4-[(4-{[(2-AMINO-4-OXO-3,4-DIHYDROQUINAZOLIN-6-YL)METHYL]AMINO}BENZOYL)AMINO]BUTANOIC 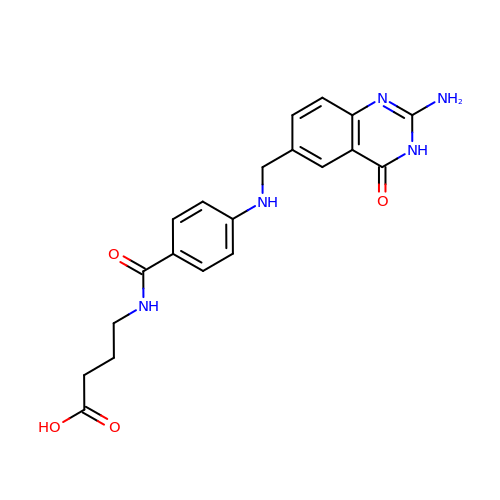ACID | C20 H21 N5 O4 | YOIMGYLREAGVGB-UHFFFAOYSA-N> KYKCGLPQPCPEEHLSFRIVSGAANVIGPKICLEDK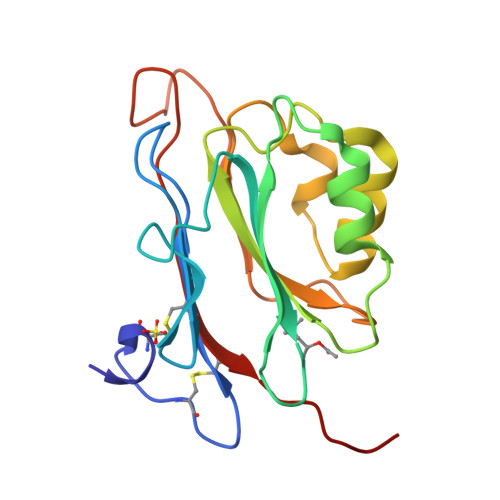MLMSSVKDNVGRGLNIALVNGVSGELLEARAFDMWAGDVNDLLKFIRPLHEGTLVFVASYDDPATKMNEETRKLFSELGSRNAKDLAFRDSWVFVGAKGVQNKSPFEQHMKNSKHTNKYEGWPEALEMEGCIPRRSIAG>NDDIEVESDADKRAHHNALERKRRDHIKDSFHSLRDSVPSLQGEKASRAQILDKATEYIQYMRRKNHTHQQDIDDLKRQN[2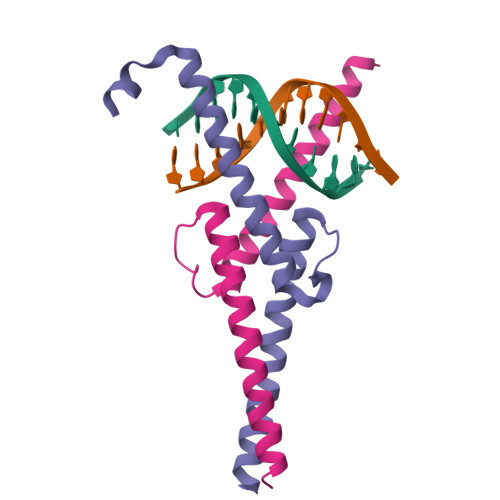x]>SLSTGCYMVKQGPTSVAYVEVNNNSMLNVGKYTLADGGGNAFDVAVIFAANINYDTGTKTAYLHFNENVQRVLDNAVTQIRPLQQQGIKVLLSVLGNHQGAGFANFPSQQAASAFAKQLSDAVAKYGLDGVDFDDEYAEYGNNGTAQPNDSSFVHLVTALRANMPDKIISLYNIGPAASRLSYGGVDVSDKFDYAWNPYYGTWQVPGIALPKAQLSPAAVEIGRTSRSTVADLARRTVDEGYGVYLTYNLDGGDRTADVSAFTRELYGSEAVRTPHHHHHH[4x]

By engineering a protein that dimerized through a highly solvent exposed disulfide bond, a system is created where disulfide bond breakage leading to monomerization is easily measured by SAXS. In this way, SAXS was able to follow a residue specific rather than a global damage process and link damage pathways seen crystallographically to those occurring in solution with much lower X-ray doses. The X-ray radiation induced dimer to monomer transition was pH dependent, suggesting mechanistic processes, routes for further interrogation, and mitigation strategies. Here, our system is engineered so that the reduction in scattered intensity is from the dimer to monomer transition through disulfide bond cleavage, making a global damage indicator into a residue specific one.

Comparison of the elution profile of endoHCYS in size-exclusion (SEC) chromatography shows that transient disulfide bond formation leads to dimerization in approximately 75% of endoHCYS (60 kDa theoretical, 53 kDa experimental) in solution. The protein crystallized in space group P21221 with four monomers in the asymmetric unit. The monomers have an average RMSD 0.289 +/- 0.016 Å to the original monomeric structure, indicating that the cysteine containing fragment did not affect folding. The cysteine containing fragment and disulfide bond are un-resolved in the electron density but is not unexpected due to the deliberate placement of the disulfides in an accessible and already flexible region. The position of the N-terminus indicates that the disulfide linked dimer forms between monomers across adjacent asymmetric units, yielding dimers with chains AA', BB', CD', and C'D. This arrangement with the N-terminus of adjacent monomers positioned in close proximity is not seen in crystal structures of monomeric endoH. The distance between the modeled N-terminal Val-8 on partnered monomers (13 Å for BB' and AA', 7 Å for both CD dimers) is such that the length of the introduced fragment can satisfy the gap and connect the monomers. Aligning the dimers shows slight differences in the inter-monomer orientation, which is most likely due to crystal packing. A PISA analysis of the interfaces within the asymmetric unit suggests that there are too few interactions between crystal packing oligomers to for those interactions to form in solution. The difference in the location of isoscattering point in calculated and experimental scattering curves suggests that the conformation of the dimer is different in solution, perhaps through freedom crystal lattice restrains to rotate around the flexible linker.> MKTFIFLALLGAAVAFPVDDDDKIVGGYTCGANTVPYQVSLNSGYHFCGGSLINSQWVVSAAHCYKSGIQVRLGEDN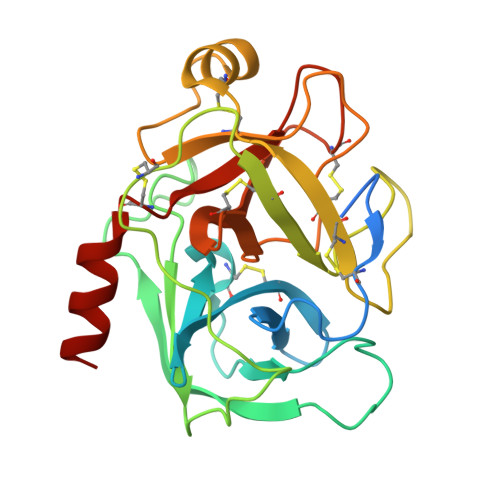INVVEGNEQFISASKSIVHPSYNSNTLNNDIMLIKLKSAASLNSRVASISLPTSCASAGTQCLISGWGNTKSSGTSYPDVLKCLKAPILSDSSCKSAYPGQITSNMFCAGYLEGGKDSCQGDSGGPVVCSGKLQGIVSWGSGCAQKNKPGVYTKVCNYVSWIKQTIASN> MSVTTETTAGAAAGSDAIVDLRGMWVGVAGLNIFYLIVRIYEQIYGWRAGLDSFAPEFQTYWLSILWTEIPLELVSGLALAGWLWKTRDRNVDAVAPREELRRHVVLVEWLVVYAVAIYWGASFFTEQDGTWHMTVIRDTDFTPSHIIEFYMSYPIYSI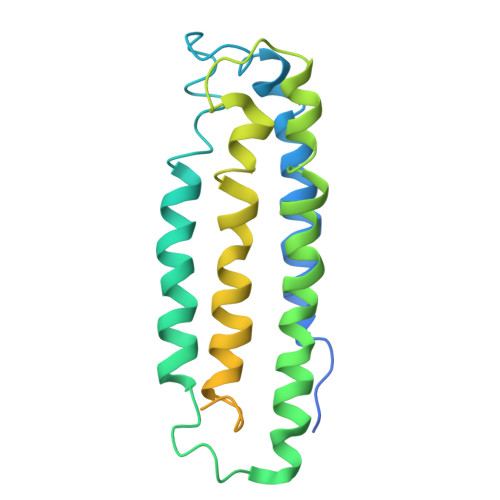MAVGAFFYAKTRIPYFAHGFSLAFLIVAIGPFMIIPNVGLNEWGHTFWFMEELFVAPLHWGFVFFGWMALGVFGVVLQILMGVKRLIGKDCVAALVG>GAMAEGELGIVDIGALTLESGAVIDNVQIAVERWGELSPSRDNVVVVLHALTGDSHVAGPAGPNYPTPGWWDGVVGPGAAIDTRRWCAIATNVLGGCRGSTGPGSLHPDGKAWGSRFPAVTVRDQVRADLAALNAMGIHQVAAVVGGSMGGARALEWVIGHPETVRAGLILAVGARATADQIGTQSTQVAAIKADPNWQNGDYYGTGLKPDVGLQIARRFAHLTYRGEVELDTRFGNAPQDDENPLLGGRYAVESYLEYQGRKLVDRFDAGTYVTLTDSLSSHDVGRGRGGVEAALRSCEVPVVVGGFTSDRLYPLRLQEELAELMPGCRGLNVVESIYGHDGFLIETEAVGKLIRQTLELAS[2x]

MetX (previously mis-annotated as MetA in the reference genome of M. tuberculosis) is an l-homoserine O-acetyltransferase, commonly also referred to as a homoserine transacetylase (HTA) and is a crucial enzyme in the biosynthesis of methionine and threonine. Here we report the structures of three homologous MetX enzymes from Mycobacterium tuberculosis (MtMetX), Mycolicibacterium abscessus (MaMetX), and Mycolicibacterium hassiacum (MhMetX) and compare them to previously solved structures of HTAs in order to begin development of selective inhibitors of MtMetX via a structure-based approach. Two copies of each monomer exist in the asymmetric unit of all three structures. MetX can be divided into two distinct structural domains, the catalytic domain, and the lid domain. The organization of the catalytic domains’ fold marks MetX as members of the α/β-hydrolase super-family.

The three solved MetX structures include residues 15–70, 77–372 from MhMetX, 10–379 from MaMetX, and 7–372 from MtMetX. The catalytic domain comprises residues 15–181, 297–372 of MhMetX, residues 17–183, 304–379 of MaMetX and residues 17–181, 311–372 of MtMetX. For MtHTA and MhHTA, Ser157, Asp320, and His350 comprise the active site; MaHTA’s triad is comprised of Ser160, Asp327, His357. Thr61/61/64, Arg227/227/230, Tyr234/234/237, and Asp351/351/358 for MhMetX, MtMetX, and MaMetX respectively all surround the active site to help facilitate the binding of acetyl-CoA and homoserine. The extended loop between β3 and β4 show differences in secondary structure content, length, and orientation. Both MhMetX and HiHTA contain a short sequence with helical propensity adjacent to β4. Temperature factors of the equivalent rings in MhMetX is B = 19 Å2, while both MtMetX and MaMetX are B = 21 Å2, values very similar to the HiHTA structure with B = 16 Å2. All three solved MetX have a similar, conserved hydrophobic patch running along the inside of the active site tunnel. All three solved structures crystallized as dimers at the expected interface and orientation that corresponds to predicted physiologically active assembly.> VAIRNFDISKISGEWYSIFLASDVKEKIEENGSMRVFVDVIRALDNSSLYAEYQTKVNGECTEFPMVFDKTEEDGVYSLNYDGYNVFRISEFENDEHIILY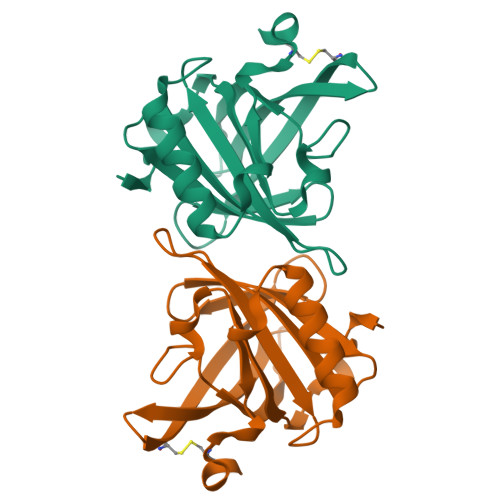LVNFDKDRPFQLFEFYAREPDVSPEIKEEFVKIVQKRGIVKENIIDLTKIDRCFQLRG> SSQIRQNYSTEVEAAVNRLVNLYLRASYTYLSLGFYFDRDDVALEGVCHFFRQLAQQKRQGAERLLKMQNQRGGRALFQDLQKPSQDEWG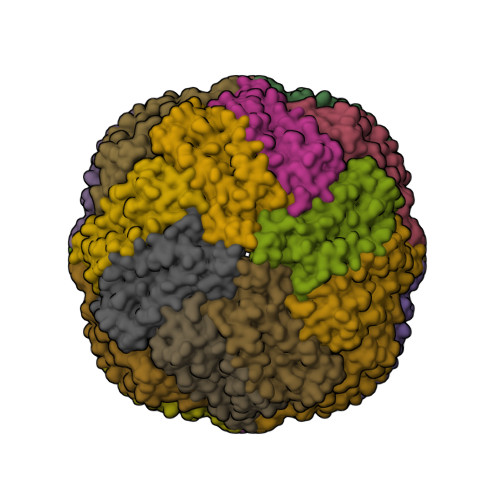TTPDAMKAAIVLEKSLNQALLDLHALGSAQADPHLCDFLESHFLDEEVKLIKKMGDHLTNIQRLVGSQAGLGEYLFERLTLKHD>[6x]MSLWRQTPDLEQLNASQKNSIGDLLGIRFEAFDDESLTASMPVDSRTHQPFGLLHGGASVVLAESLGS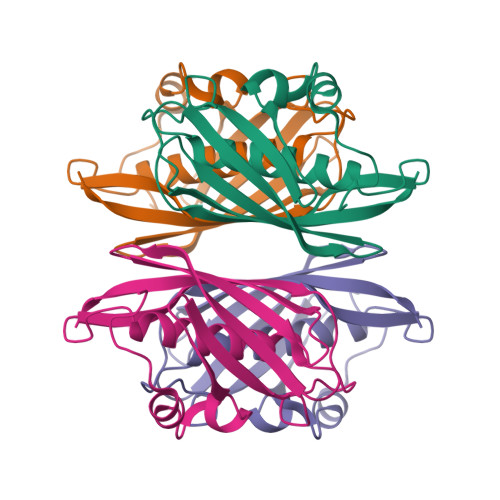MASYLCVDTSQYYCVGLEVNANHLRGLRSGRVTAVARAIHLGRTTHVWDIRLSGDDGKPSCIARLTMAVVPLAGRALEHHHHHH>[4x]MTVVPENFVPGLDGVVAFTTEIAEPDKDGGALRYRGVDIEDLVSQRVTFGDVWALLVDGNFGSGLPPAEPFPLPIHSGDVRVDVQAGLAMLAPIWGYAPLLDIDDATARQQLARASVMALSYVAQSARGIYQPAVPQRIIDECSTVTARFMTRWQGEPDPRHIEAIDAYWVSAAEHGMNASTFTARVIASTGADVAAALSGAIGAMSGPLHGGAPARVLPM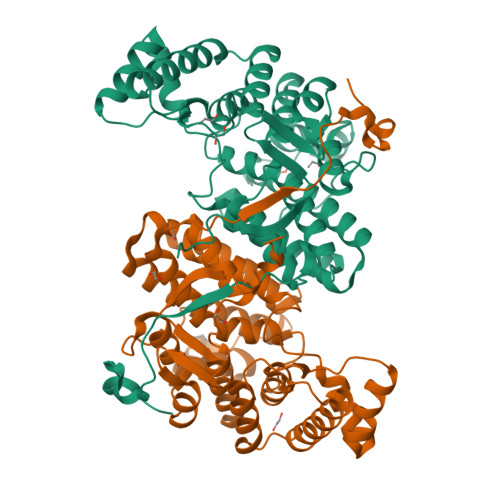LDEVERAGDARSVVKGILDRGEKLMGFGHRVYRAEDPRARVLRAAAERLGAPRYEVAVAVEQAALSELRERRPDRAIETNVEFWAAVVLDFARVPANMMPAMFTCGRTAGWCAHILEQKRLGKLVRPSAIYVGPGPRSPESVDGWERVLTTAHHHHHH>MQAEKLGSEIKKIRVLRGLTQKQLSENICHQSEVSRIESGAVYPSMDILQGIAAKLQIPIIHFYEVLIYSDIERKKQFKDQVIMLCKQKRYKEIYNKVWNELKKEEYHPEFQQFLQWQYY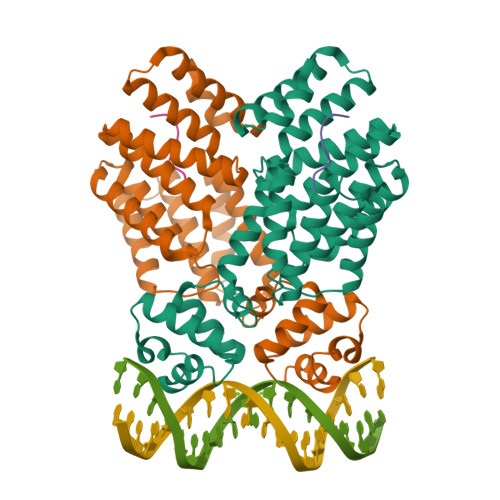VAAYVLKKVDYEYCILELKKLLNQQLTGIDVYQNLYIENAIANIYAENGYLKKGIDLFEQILKQLEALHDNEEFDVKVRYNHAKALYLDSRYEESLYQVNKAIEISCRINSMALIGQLYYQRGECLRKLEYEEAEIEDAYKKASFFFDILEMHAYKEALVNKISRLEHHHHHH[2x];>[2x]ADLPFEF5-[1-(4-methoxyphenyl)cyclopropyl]-1',3'-dimethyl-1'H,2H-3,4'-bipyrazole 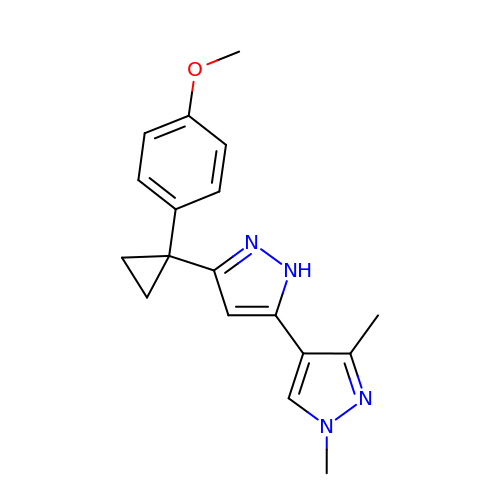| C18 H20 N4 O | ZLBUFDZQBDNLRH-UHFFFAOYSA-N> MTVTAPNALNFECETGNYHTFCPISCVAWLYQKIEDSFFLVIGTKTCGYFLQNAMGVMIFAEPRYAMAELEEGDISAQLNDYEELKRLCLEIKRDRNPSVIVWIGTCTTEIIKMDLEGLAPKLEAEIGIPIVVARANGLDYAFTQGEDTVLAAMAARCPTSTAISDPEERNPIQRLLNFGKKKEEVQAQSSQYHPHPPLVLFGSLPDPVVTQLTLELKKQGIKVSGWLPAKRYTELPVIDEGYYVAGVNPFLSRTATTLIRRRKCQLITAPFPIGPDGTRTWIEQICATFGIQPQGLAEREAETWQKLSDYLELVRGKSVFFMGDNLLEISLARFLIRCGMRVLEIGIPYMDKRYQAAELALLSQTCAEMGHPLPTIVEKPDNYNQLQRIKALQPDLVITGMAHANPLEARGISTKWSVEFTFAQIHGFGNARDILELVTRPLRRNQALAGLGWQKLVAH;> AAAMKLAYWMYAGPAHIGTLRIASSFKNVHGIMHAPLGDDYFNVMRSMLERERDFTPVTASIVDRHVLARGSQEKVV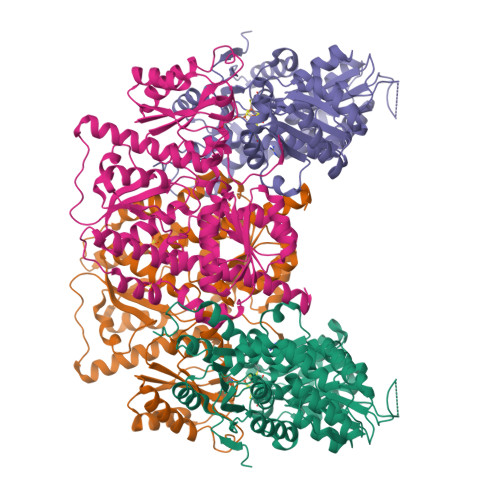DNIIRKDTEEHPDLIVLTPTCTSSILQEDLQNFVRRASLSTTADVLLADVNHYRVNELQAADRTLEQIVQFYIDKARRQGTLGTSKTPTPSVNIIGITTLGFHNQHDCRELKQLMADLGIQVNLVIPAAATVHDLQRLPQAWFNLVPYREIGGLTAQYLEREFGQPSVRITPMGVVETARCIRAIQGVLNAQGAGVNYEAFIEQQTREVSQAAWFSRSIDCQNLTGKKAVVFGDNTHAAAMTKILSREMGIHVVWAGTYCKYDADWFRAEVAGFCDEVLITDDHTVVGDAIARVEPAAIFGTQMERHVGKRLNIPCGVIAAPIHIQDFPVGYRPFLGYEGTNQLVDLIYNSFTLGMEDHLLEIFGGHDTKAVIHKGLSADSDLTWTAAGLAELNKIPGFVRGKVKRNTEKFAREQGISEITVEVLYAAKEAVGA>CUGGGCGG[2x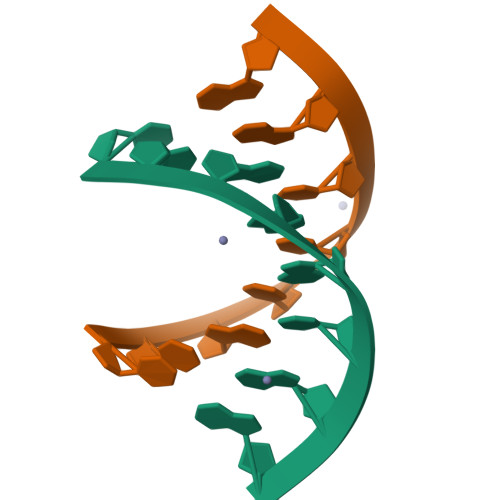];>[2x]CCGCCUGG>[2x]MYETIRYEVKGQVAWLTLNRPDQLNAFTEQMNAEVTKALKQAGADPNVRCVVITGAGRAFCAGEDLSGVTEEMDHGDVLRSRYAPMMKALHHLEKPVVAAVNGAAAGAGMSLALACDFRLLSEKASFAPAFIHVGLVPDAGHLYYLPRLVGRAKALELAVLGEKVTAEEAAALGLATKVIPLSDWEEEVKQFAERLSAMPTKAIGLIKRLLRESEETTFDRYLE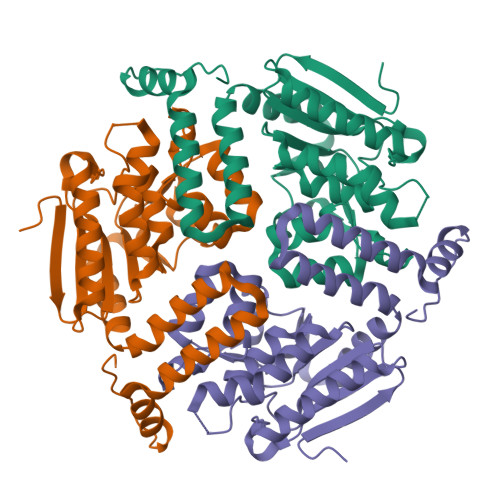REAECQRIAGLTSDHREGVKAFFEKRKPLFQGN>GSSPSLEQDDGDEETSVVIVGKISFCPKDVLGHGAEGTIVYRGMFDNRDVAVKRILPECFSFADREVQLLRESDEHPNVIRYFCTEKDRQFQYIAIELCAATLQEYVEQKDFAHLGLEPITLLQQTTSGLAHLHSLNIVHRDLKPHNILISMPNAHGKIKAMISDFGLCKKLAVGRHSFSRRSGVPGTEGWIAPEMLSEDCKENPTYTVDIFSAGCVFYYVISEGSHPFGKSLQRQANILLGACSLDCLHPEKHEDVIARELI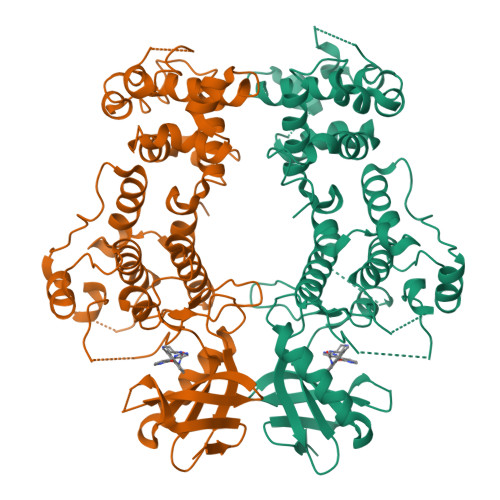EKMIAMDPQKRPSAKHVLKHPFFWSLEKQLQFFQDVSDRIEKESLDGPIVKQLERGGRAVVKMDWRENITVPLQTDLRKFRTYKGGSVRDLLRAMRNKKHHYRELPAEVRETLGSLPDDFVCYFTSRFPHLLAHTYRAMELCSHERLFQPYYFHEPPEPQPPVTPDALGNS[2x]> ASSGPAAPDATHSTHAARPASAASSTSPMNPTSTPGASGPAHAKAALDAARAKAAPPSPPTTVLLPGAPPERVVDTIGRGTPQVASKVDPTAAVFRPDPTLAALGKRVFFDPALSEPRGMSCASCHDPGRAFAPTLSPAALAGPRVPQGSRPGHFSRRNAPSLLYVRYVPRRHFYQDDDALAPAPFGGLFSDGRADTLAEQLRGPLFDPDEMNNASAAALMRKIGRTGLGAALAGRFGPSVRRDPERMVRVLGEAMQAYLQSDEMAPFSSRYDAYVTKRAPLTPQEMRGLALFRNPDKGNCMSCHTLSDTASRPERSLFTDFGYDAIAVPRNRALPANRDPRHFDNGLCDTAAKLRWPEPTQWCAYLRTPGLRNVAIKESFMHNGVFDTLRDAVAFYNTRSTDPARWYHGRDTFDDVPRAYRGNVNVNSTPMNRRPGTPPAMTDADVDDLVAF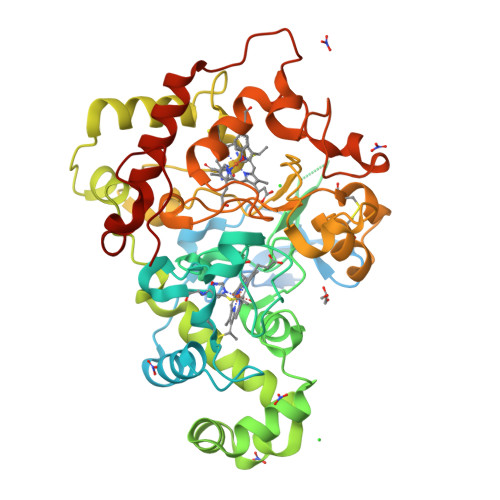LRTLTDARYVGLMPTAPDGKAARP> FKTRMRSTVSVREGQGVVLLCGPPPHSGELSYAWVFNEYPSFVEEDSRRFVSQETGHLYIAKVEPSD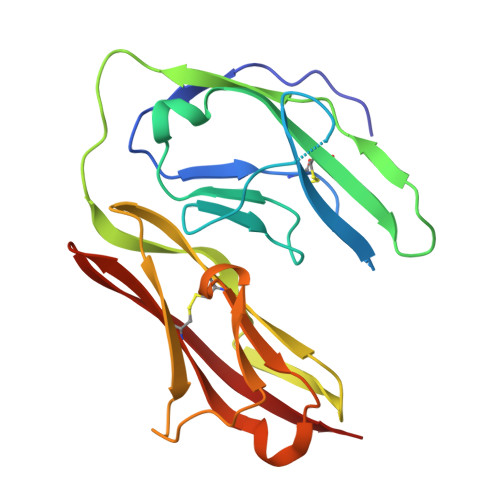VGNYTCVVTSTVTNTRVLGSPTPLVLRSDGVMGEYEPKIEVQFPETLPAAKGSTVRLECFALGNPVPQINWRRSDGMPFPNKIKLRKFNGMLEIQNFQQEDTGSYECIAENSRGKNVARGRLTYYA> EKNSKDAQKMINEMQKRNRQTNERIEEIIRTTGKENAKYLIEKIKLHDMQEGKCLYSLEAIPLEDLLNNPFNYEVDHIIPRSVSFDNSFNNKVLVKQEENSKKGNRTPFQYLSSSDSKISYETFKKHILNLAKGKGRISKTKKEYLLEERDINRFSVQKDFINRNL;> MKSVKYISNMSKQEKGYRVYVNVVNEDTDKGFLFPSVPKEVIENDKIDELFNFEHHKPYVQKAKSRYDKNGIGYKIVQLDEG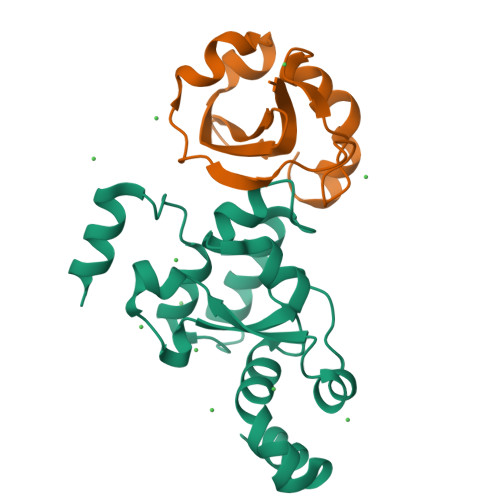FQKFIELNKEKMKENLDY> GSHMTIQKVHGREVLDSRGNPTVEVEVTTEKGVFRSAVPSGASTGVYEACELRDGDKKRYVGKGCLQAVKNVNEVIGPALIGRDELKQEELDTLMLRLDGTPNKGKLGANAILGCSMAISKAAAAAKGVPLYRYLASLAGTKELRLPVPCFNVINGGKHAGNALPFQEFMIAPVKATSFSEALRMGSEVYHSLRGIIKKKYGQDAVNVGDEGGFAPPIKDINEPLPILMEAIEEAGHRGKFAICMDCAASETYDEKKQQYNLTFKSPEPTWVTAEQLRETYCKWAHDYPIVSIEDPYDQDDFAGFAGITEALKGKTQIVGDDLTVTNTERIKMAIEKKACNSLLLKINQIGTISEAIASSKLCMENGWSVMVSHRSGETEDTYIADLVVA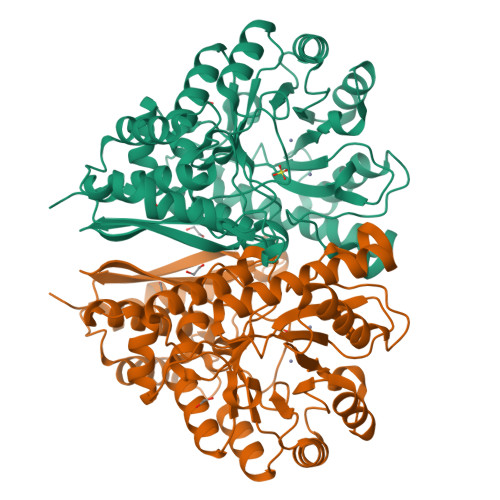LGSGQIKTGAPCRGERTAKLNQLLRIEEELGAHAKFGFPGWS>KNAPSTAGLGYGSWEIDPKDLTFLKELGT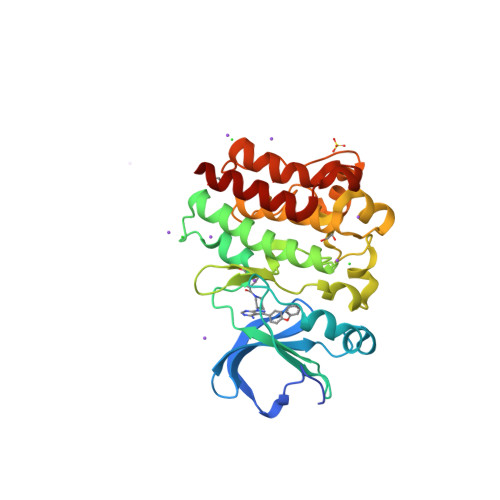GQFGVVKYGKWRGQYDVAIKMIKEGSMSEDEFIEEAKVMMNLSHEKLVQLYGVCTKQRPIFIITEYMANGCLLNYLREMRHRFQTQQLLEMCKDVCEAMEYLESKQFLHRDLAARNCLVNDQGVVKVSDFGLSRYVLDDEYTSSVGSKFPVRWSPPEVLMYSKFSSKSDIWAFGVLMWEIYSLGKMPYERFTNSETAEHIAQGLRLYRPHLASEKVYTIMYSCWHEKADERPTFKILLSNILDVMDEES[2x]>[3x]MNDQTQFTERALTILTLAQKLASDHQHPQLQPIHILAAFIETPEDGSVPYLQNLIEKGRYDYDLFKKVVNRNLVRIPQQQPAPAEITPSYA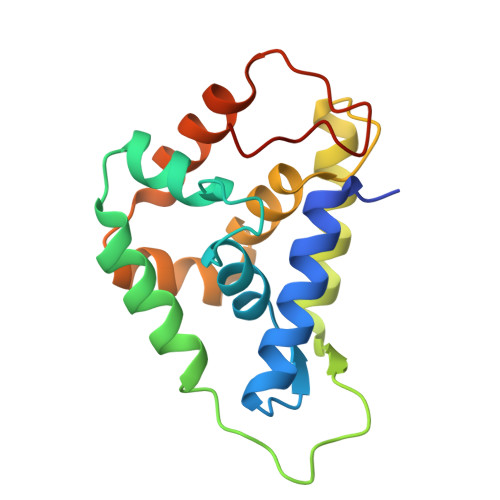LGKVLQDAAKIQKQQKDSFIAQDHILFALFNDSSIQQIFKEAQVDIEAIKQQALELRGNTRIDSRGADTNTPLEY> GSHMASMNYEIEVKDVEPIRVAFMHYKGPAAGASKVMPNVFKSIQGKANGAPFICYYVMDQQTMTGEMDLCVPTAENPVGNGIAVKDMPRIKAISATHIGPYETMQPVYEAIESYAREKNLILQPPFREVFIKGPGMILKGNPNKYITEVLFPI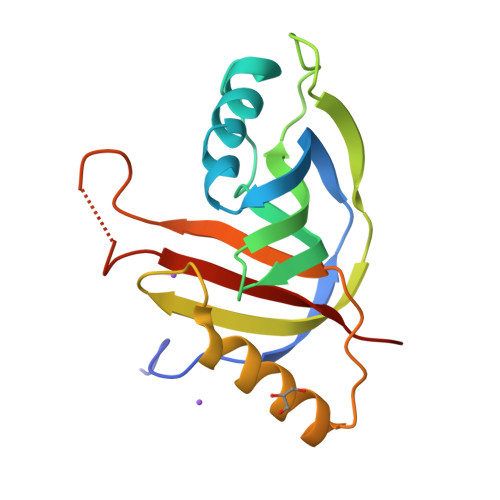KEEC> MDGEEVKEKIRRYIMEDLIGPSAKEDELDDQTPLLEWGILNSMNIVKLMVYIRDEMGVSIPSTHITGKYFKDLNAISRTVEQLKAESAL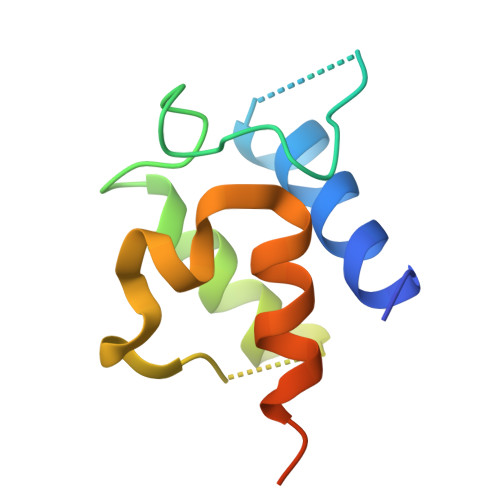EHHHHHH> MPQPLVWTQLKQTGTTQPTARSGHTIITVGKTHIMFGGLDNDKNNYKDGKIAPNNQVFTLKLTQNNCEWRQIACQGDVPLPRCYHASCAISADKMLVFGGSYTSNLRFNDTYILKTTSYQWSKPANQISGGEPKNAESKIGAPQPRYGHSATFFEGKVYIFGGHGGINYQRLAFNDLYVLETENFEWTRLEPKGNPPDPRGGHSAAMMANKPQLMIFGGWSFTSQYSNIMIYDIEKDEWVDPEIAHEIPKWNLSGIMAPSIPSWKYFIFGGSVGSFEEGGNRTNSRFVDDSFVLDIDTLSWSSINLEADETSKAVCKPRPRESASIFYDSGESRAIVFGGWANNWLNDLWALNVSTITGPPYAIFSIKPALGPLTGKTKVLIEGDGFKDTQNISVKFSGGKLEKEVNGTFVNEKEISCETPTFDYPRSVEVTVCMNKGDYTITKSAFTYYLNTKADKTIAYGPGLLTENLIGVQTTIVIQARNKNDQNRESGSDEFVVTIRNPAKIKKEEEVKEGDKANTKNTIKEDEEEEGEDEEENKKKKEAEKAAAEKAAAEKAAEEEQGEAVDPSLVPFNIVDNDDGSYFIQFTSEEEAVLEIDIKFKDENNELHSIRGNPFRCGFVKGSKPNNNDLTGSAVMNYISKQLKDIQEFIENTKENIEIRNKNIRENVSELINVMINLEKVRVKNDDDVLTLDTVEEMLNFLKKKDFGKDSDIKKCKKLQEEWKNLAKMAQAVKKDIQNPVKTESDKTKENIKKFEEITLKEYANSLKKESFFIYKTGVSESFKRIGEVKQKVDEFEVQLNQYEDFARMFEFPDAVIGSKKLMEQIRTDVSSVEKLWVRIEISEKTMDEYKKMKWGSINSMDMEDEIKKLRKALTDLRGIDKRSNAFIGITEELKKWATFLPLLGELKDPSMNSEDGRHWKKLKDLVKKEFDVSQELMLEIIWDLKLFDYKDGIEEITDQAKQELKMEKALKKIIDFWRDIEFELVQHKNTDIHTLKMSEENFETLEDHQLQINNMLLSKYVAYFEKEVEKWKYDLGSVYDVVQLLLEVQKTWSFLENLFIQSEEVKRELPNESAQFVGIDKDMKEIMQKGCDIKNCLKFCTIEGMLKRLENIQAQLKVCEKALNEFLDSKRRAFPRFYFVSVNDLLDILSNGNSPAKINRHMSKIFQAIDNLQLKEDSSGGRPTALKMISCVGTEEVDFSSPRLLQGKVESYLKDVIDTMIGTLKSVANSSFKNFQSMTRKEWLKSDPSQITLLVNNIIWSKAVEDCFLKLQSGDINAMKLFLDESIKQLTELIGMVQGDLSKPLRQKIMCLITIDTHSRDVVHRLINEHVRKAEEFQWQSQLKFYWVDNDAKIKIADARFVYNYEYLGNGPRLVITPLTDRIYVTATQALHLKMGCAPAGPAGTGKTETTKDLANALAKACYVFNCSSEMNYESMGNIYKGLASSGCWGCFDEFNRLLPEVLSVCSVQFKAVTDAIKQNVERFIIEGDEISLDPTCGVFITMNPGYLGRAELPEGLKALFRPITVVVPDLELICENMLMAEGFIEAKILAKKFVTLYMLCRDLLSKQLHYDWGLRAIKSVLVVAGGFKRSEPEIAEQALLMRALRDFNIPKIAFQDLYVFHGLLGDLFPGINIKPKKDLDFEKIITDVCIENKLDPDPEFVLKVVQLSELLAIRHCVFVMGPPGAGKSTTWKILAKAQDKTNKKTTLIDIDPKVVSTKDFYGYNLPSKEWKDGLFSKMLRSLAEQPDTNPKWICLDGDLDANWIESMNSVMDDNKILTLANNERIPLKPHMRALFEIRDLRFATPATVSRAGILYISDEVGYQWRSYVKSWIKQEFSQDQEMSKNLDTLFGKYVPDTLDHIKKHCRFLVPVSPISQVISICKSLQTLLKGDVKNLEYLFVYALIWAIGGALAEKDSIDYRKDFSTWWKGAWKTAVKFPSKGTIFDYYVDQSGDSSKFVEWSKRLENKEFDPQVETMGNITVNTIETLATTEFIKSYLMVKHPSLLIGNSGCGKTQLAKGILKEIVQAKPENYAYQLINFNYYTDSTYLQGQIEQTLEKKAGRQYGPPGKVQLIYFIDDLNMPQLDAYDTQTAIALLRQLADYGHFYDVSKLALKDIINTQVLAAMNPSAGSFFVNPRYQRHFWTISIPFPDNESLSLIYITFLNGHLKRFKSTIQEYSNIIVRASLMLHQAVTQNFRKTAINFHYEFNLRHMSNVFQGLLLSDPNKFTEPDKLIKLWIHECERTYGDRLVSTDNLKTYKENIFDIVKKSFSKFNFSRYFGNNPENLIYCNFIAGINSDRFYDQMPNNEMEKHISEALKEYNDNNAFMGLVLFEDAMKHVCRICRIVLPSSGHALLVGVGGSGKQSLSKLASFIMGYTTFSITISATYSMVDLRNDLQQLYFKCGPKEEGILFLFTEGQITNERFLVYINDLLSSGEIAELYTLDEKEAMINQVRAKVKGEGKPDTRENCWNWFIDQVKKNLHMAICFSPVGDMRRRARQFPALVNCTVIDWFQPWPYEALFNVAKSFLEPVDLGDDKVREAVVKFMPFSFTLVNDLGLKLLEQERRYAYTTPKSFLELISLFTNMLAQKRESLERNKERYETGLVKLKETAEQVAIIEVEVKEKQVEAEAKKKEADAFAEVVGREKDKVEKENSKATIEADKCGLIKQNVEAQKSSTQQDLDAAQPLVEQAKSALNSISKKDFQQAKSFASPPAGVPEVFAATIYLLAGYFNEAIEIDKNKKPKDVSWKSSLKLMKSPEEFMEKLLNFKDVVDANQVPAANVNIVKNQYLNMPSFTPEQMASKSAAAKGICSWVVNIVKYYDVIQDVEPKRKALKEATEQLEEATVKLNEVEEVVRKLNEELNKLKAENDKAIAERNAAISEAERCARRLNLAQRLVTALSSENERWGKSIIQLEDQLKLMVGDVLVASSFVSYSGPFNKKFRNIMINQNFMKFMKEHTIPMSPDPNPIKILTDESTIALWNKQKLPSDSVSIENGTILTNSARYPLMIDPQLQGITWIREKEKANNLKILRLGSKNINRDLELSIENGYSAIIENMNERIDAILMPIIARSFIKRGKNKIIKFAGKDLILHPNFKLFLHTKLSNPHYPPEIQAEAALINFTVTEAGLGDQLLSLVVARERPDLAKMKIELITQQNDFKIKLKDLEDELLYKLANAKGDILDDIELIENLEYSKKLSVEIAEKVAAAKITEAKINETSENYRPAASRGALFYFLLSDLSKVHSFYKYSLESFIVVINRAIDAISENKIYGKTTMVPYGDETYASNQHEKEEEEEEEEHQQAQQQQNQEEQQEQKDEENKGPVEEEQPEGENKGPVEEEGAEGQNEGPVEEENAENQEGEGEEEGEKQQKAKDSDEPMSPRSLKKRVDELIESLTYTAYQTTRRGLFESHKLIVAAMLCLRVLLRSEELNSDEVDHLIIGKVDVNPTPMPDALKSFLNDNIWAACKALETIHQFQGFCQSLETDVLQWKKWYSEEKAETADLPKAFKELSKFHRLLLLRALRPDRLPSALSQFVHDKMGERYIEQPPFNIFETFQETSKTVPIFFVLFPGVDPTPDVERVAATFDVSANNGRFINISMGQGQEDRAKKALFDCAQKGHWIMLQNVHLMQSWLYGLNGLEGFLESVFASPKTHPNFRVFISSEPPNVLLPLMQIIPESILQGSLKIANEAPQYLKANLRRAYNKFDQEFLDKCDKKPTEFKSCLFALCFFHSLMLGRKKFGTQGWSRVYNFNDGDLTICADVLYNYLSKYDQVPWDDLRYIFGEIMYGGHITDDWDRRTNRTYLKVLIRSELLQQNFNLAPQFKSPDPSKFDYEAYRKYIEEKLPIESPQMFGMHPNAEIGYLTQTCDQVFNTILEVQGGSSGGGASKKDDGVMVTLTDFKTRCPHDFNMLLIEEKVKEKTPYIVVCLQECERMNGLLKEIKTSLEDLRLGLTGALNMTDAMESLQQSLSFNKVPDTWEKKAYFSKKPLSSWFADLIERNIQLQEWCKELVTPTSLCISYLFNPMSYLTAIMQFTARAQGLPLDGITIQTNVTAMKGPEDVVNPAENGAYIHGLFLEGAAWEIGGQGQDGYLIEQKPKELHPKMPVINAVAVPLDKKKKNGQYDCPTYVTSARGQTFVFTANLNMESDDSDPNKWILSGTCMLMSDD;> MGDHSQKDSPEDFIINRLSQALGIQKEKIKKSLETQQDDKGEVTNKDEFQGFIQQDNSTNILWVSGQSEKCTFYYGQLPPIDKFKKKGIAVIKLGLHKLTNENVAKDVVVVEITNNLLEHLNSVFNEIMSPVMQNPLNQQGWTDLVAKDLMEKFNNYVAQVYVLLGQIKGKTMLPLPSHKLTSSDTTPDKDKAHVFEGSIITWTKQIKNVLKLEPEQLLKYGNDPGPLAEIEFWQNKRDNLNLIDSQLKSVEVQNILHFLDNNKSTYTTPFTKLQAEVKKARLEANENYRYLFTLKDLFSKLQESQPSDFPTLYELFIPIMHTILLIYNKSKTYNQPPRLVVLIREICNAIISNAQAFVDKDTIFSLIDSKETTEACDKLQVTLDVCSKFKDAYFEYKAKAGGNWKLTSNALFVRLDSFLERCQDILHLTNTIVQFNKLEKIELGGTKGKTLTESIAQIFKEFEEAVQAFTSVSYDIMNIAEKKFDDDFYEFRSKIKELERRLASVITQGFDDYDTIYGRFKLLDNFEGLLTRPIIADELEKKHIVLLEMYKQDLKQVQSIFLEGKQFVDSMHENAPLFLNMPPIAGALTWCKSLRDRIQEPIEKLAQLGQGITEREEYKDVQKLYTSITKSIKDYEDQKILSWEKEVEDSSQDKLKQTLLCKDENDLIKVNFDPSLVRLLKEVKYFLLLRLEVPTTAKDIYTKAETYRTQIVALDMIVDNYNHIKTCLLPVEEPLVKKKIQDMEEEVKPGIEEIRWKSTNIDQFISKSKSIVDQLFETVNKMKDSLQKIHKSLANFNVKIIERKNRPMSPDDYDQFLKAIFSNKLTIVKDNGNQIQKLVKEVLDAVKADKKQNSWKNYNDYVNVIVIEGISTAIQTALLHLNEQINPVFIKRNDISPLFDIRLELGQSGIQFDPEIGESSNQLTVRNTIRNWINDFFNIAGTIQRLDTTMPGDFLQEIRSFFEIKQCLAMITQNLEWIENECNQFRARFDTYSYLWTEDEQISFNRFLDENEPKDEDGKGGDDDEGENTEKQNPLLKGCRAKIPNLDLFDEKITHLKAIQQEISRIKTPEDISWLRINLQPMKTALDARVTRWIRVYTDFLVNQFRTTQKNLLDFIEKTKDGIKKNPADHENLHDKKLLMSVMKVISDVKDVEPRREGIITRMKEMVTKLKKHNVPITEKGTDDPLQQIDNANSNFIEIYGRVFKVKADIIPLQAEETQNIKRDLDIFMKEVESFRKEFMQKLPFDYTESMGYENINNAYDTIMVYYHKLTAIEGRALEYNNLEKLFELQKSNYKQLKDCMNDLKNLKTMWDAIALIHFQYNDWKTKPWRQIKADILLDTNKTLGTQIKNLPKEIRNFKGYNVIVEKVKNMGTVLPLVSALHSEFMEDRHWSQLKQITGTVFDHNSLSFYFEDILALNLYKYENTVNEIVDVAQKEAKIEKKLKNIEQWWSKQVFEFTEYKETKTFASLDNMMEVLDQHSLDLMGMKSQGKYVEFFYDRVEDWREKLGRVDVVVNEWLKVQKNWKILYNIFLLSEDIRMQLPEDTKVFEGVDKEFKDMMSEVSANPSVVEACTIERRDVLVGWSQAIKKCEKALNDYLEQKKKSFPRFYFLSNQSLLTILSNGQNAPKVCEYLGDCFDGLKTLTFEPPANPAETSKVGIGMISKDDEKVPFSSKFICEGAVEHWLLNLEFRMRETLQEILEGAKNTADLWDSGDKPREEWVEGYNAQIALLTTTIVWTEDVGRAFEDLAGGSETAMKECQKLIEVRLENLIKKVRGDLHILERWKIINIITIDVHSRDVVEKFVIQKVSEAESFAWLSQLKFYWENKPDSDMHLRQTLRFPWEKDKNKNKCIIRIVDWFRFYSYEYIGNAIRLVITPLTDRCYITLTQALNLTMGGAPAGPAGTGKTETTKDLGRAIGIPVMVFNCSDQMNKDSMAQIFMGLSQSGAWGCFDEFNRISIEVLSVVSTQVKCVLDALKEKKTKFSFVEEGEIQLQDTVGFFITMNPGYAGRTELPENLKALFRSCAMVVPDLALICENMLMSEGFTMARVLSRKFVSLYMLSRELLSKQKHYDWGLRAVKSVLRQAGKLKRGDPDMPEDPLLMRALRDFNMPKIVTDDKVIFRRLIGDLFPKLDPPTKQNPELKKIVQDTTKKDMGLVAEELFVTKVVQLAEILEVRHCCFVIGPPGSGKTCVWKTLIKSYINSGEDAEYDTLNPKAVTSDELFGAYTKTKEWKNGVIAVIMKNQVKNEEKYKATHMHKWSVLDGDIDPEWIESLNTVMDDNKVLTLVSNDRIFLTPQMRLIFEISNLRNATPATVSRAGVLFINETDIGWMPYMNSWLERSQINILKQQKEMANMPEYPVIDDVAKSVFYRCFQSYFEQNIDVHDKNRVRHICPMVDIAMIQTICTILDALLIQHLPKLKQMKEEDEKQALEAFFIFAGLWAIGGPVGGGQDDSKDMKEFNTVWKGAAKVKFPEQGLCYDYYYDINENKWNTWKVEDYLPNDQPLFSKIYVATIHTTRLRYMIDIHLQRRKPILFIGSAGTGKTAVVRDYLNSTRPEQVSHKTINFSSFTDSLALQKNIESMVEKKNGRNYGSATNKVLICFIDDFNMPYVDKYGTQSPIQLLRLILDYGSIFNREQLEERKFLQDLLFFGCLNQKSGSFTVDLRLQRNFSVFSMYTPSSDVIKTIFGSILNAHLSTIDDKAQKMAFKLVEATYFTFDKILKNTTAFAPSAKRFHYQFNFRELARVCEGICRTTPGQYSGGDQGKLVRLWAHEMKRTFEDRFIANEHVEFFRRYLTEAISKCIGEFPETENPIAEPLIFTGFVAAHQGLDQQYTQCTIPVLKRVLDDKLEEYNEVKAQMNLVLFQQAMEHVSRICRILDMPGNNALLVGVGGSGKQSLCRLSTFINGFEIDQLVVTASFTINDLRNNLQEIYKKIAKPNSIARVFMITDSQIKEEQFLIPINDMLNSGWIFDLFPKEDMDSLVSGVRNEAKGEGVDVNNLTALTSYFLDKIRKNLKVVLCFSPVGDTMRIRSRKFPGIINNTSIDWFHPWPHEALIDVAFRFLEEIEFPTEEIRQSISLNMAKVHSSIDTANEKFLKLERRYNYTTPKSFLELIDFYKKLLTEKRETIQRQIQRYEMGLNILAETQNKVQGLQEELKVKMVEVNKQREETDILIEKVGKESALAEEEQTIANAEEEKTNVAAAEAEKISKEATEALAEALPALRSAEAAVDCLKKPHVTEMKNLGSPPAGVIVTARVVLILFNQGITLNDPDEKVWKKAVTFMNNPQAFIDKVKSFDGENIEPNIIEQSNKIIQDPSKKFNEKDMAGQSYAASKLCAWAVNIVTFNKIFKQVKPLQDAQKQANEILEEKKKELAIVKQRVAELNARVNSLKRQLEEAEARKMIVEQDAARCQSRLSAAENLVNGLAGENKRWTQNVKFLKENIKSMIGDSLLASAFVSYIGAFSAKLRLELWKNTWLPDIIEKGIPITEGIEPLKILTTEAIKSKWKNEGLPADPMSLENAAIITACARWPLIIDPQLQGSTWIRGKQGENLTTISLSQPKWLGALTSSISSGRAVLIEGIQQEIDATLDPLLQRAVKKNGNQLQLEIGGDPIDYDPNFKLFLMTKLINPHFRPEIAAQCTIINFIVTESGLEEQFIAMVVNIEKNELEMAKQDLVKKQNEYAVTLDKLESDLLQSLSEADPATILDNTELIQNLDKTKKTTIEITEQQQKAKVTEAEINIQREHYRVVAAEGSMLYFLVISLSVMDHMYQYSLESFITFFFKAINRTTVRDENRIPTLILNIRQTIYQWISRGLFEKHKLIFLTLIVFRLMQKKIIDVAYEVAEMDFLIKCPARPGVENTLDWLPNISWDQIQGLINLEEFRNFAHQLEKEAPNRFKDWYNELQPEDQKLPLDWKRLDSMPFKKLLVLRCLRPDRMTISLNNFIRAVLPQGDAFVEMDQKLAFSEILESVINEDSESTIPIFFILSPGSDPVKEVEKIAKKKRIEPGKNFFNIALGQGQDEIARRRIEEGNKEGHWVMLQNIHLMPTWLIELEKILDSYSGEAGGGNSEFRLFLSAEPSTGIPIGILDRSIKLTNEPPAGLKANMKRAWTYFSKEEIEDKDPKIKSILFALCFFHSTLIERRRFGPKGWNMSYPFNMGDLRDSYLVMNRYMEQNQGGKVPFNDLIYIFGEIMYGGHIVDDWDRRLCNSYLFNTMHEQLFDELELFPYIEGKGLSFKVPGQNPYEKYIEHIETSLKQETPLAYGLHPNAEIGFRTDQCKTLFNTLLELMPKEQSRDEKSSDIKSSNEMASDLIKQLLEDSELKNKIFNMEEIKNKIDAENKGPYQNVFLQEIEYMNALLSEIVKDLEEIGQGLSGLLTVSENMEMIIESIALSRVPASWQKLAYPSKRGLQSWLANLFQRIEQLNIFRDDPYSIPRVVMISRFFNPQSFLTAIMQVISRAKAYELNKLYIQTEITKRSIEEIEGAAKEGAYVYGFILEGARWDYQLGQLEESKPKEMFSVLPVTYCKAIPLPPEGKEDKSLYQCPVYKTEDRGNTYVFTAQLKTRFPPRKWILAGVAIIMDVEGVSDEVKKDKK;> MLSSKYSKRIAWMKTTICDSLQLKDMIVEESFQYEKNKNLLEQFLSGEGLNKIFAYYQVQEQAQNDDIKDTGAQDPVLFFTTGDLEKIQDKAVWFLRITNPADDKKKASQQDGNDNDIIFGEITPNTVPMLNALMESVYSRQIDHIITEKIQFWGVAEEEQVLEFQQHSNKFSSEVREAINLMSPGTEHFKLDYEAISGLSESEKMQHYEMKFNEWINLISSQLNDDSEVRKDEKDAGPATELIYWRSRMQKITNWSEQLKSKDFQIVKASLQRHKNHDNQRPRGDESLSKLMMEYNRLDLLLTDKLNEAKDNVKYLTTLEKFIEPLYNGTPQQIIDTLPALMNAIKMIHTIARFYNTTDKMTGLFIKITNQMIKNCKDRILNKKDNGDNPSLYKMIWEQDPAELIEVLGSCIKLYCEYKKCYNDTKEKVADMPKGKTFDFSDAQIFGKFDTFVRRLQKLIEIFSNIQQFNALAKHNLEGMDVLTNKFKKIIDDFKKKGHNLLDTANNKFDRDWVEFNVEISHLDGELQNFIDNNFNRFRNIEYSLKLLHKFQSTIKRDSLKHNLTSRYNAILHNYATELDTIQRVFQDQKSNPPLVRNMPPEAGKIIWARHLFQKITGPINIFPENVINSTEIRRYYGSYNTLGKQLTIYEMWFYQDWVNKIEQSKAALQATLIVRHDENKKLYVNFDLEIMQLIREAKCLDRQGIEIPESARIILLQEDKFKTYYNELLYALKEYERINSKIKPICKNLLLPHIEDLDLKLRPGMVTLTWTSMNIESYLYYVHQGLKKLEQLIINVNDIIENRIENNLKTVSKVVLVHLPQDTKPLSLDSFVQLQEEYINSKTDFLTSKNVEVERAVDDLLQTIMLYPLDPHVDPVLPEETKRIKRYYFWYFYQALLNSTQNSLNAMKYRVCGKKIPGANTLQNLKPFFQVEVQLNGDKVTLNPSLQEIQKSINRAATAVLRCSKHLYNWDQQNKDSTDKATFYDMIACDKEIVKVILLLTGSIQGTKNKVNEFLSGFTKFEWLCKESIQESIKKFSKNGPTLQNYEDQLKKFSQIEEEIEKIVPTYKIGAMELMTHNICTSLSTWAKEWKLQYSQDLHKRARQLLDSLTEQTKMLSTKLSKPVKDIDSLGYVMETLEQIRKEQAEIDMKFNPVQEMYSLLDNYLPGGITDKDEMDARSLLRRNWDILIQQAEIKGKEYQHKQAIYLKELKQSIKDFTNQVSIFRRDYEKNGPMVEGISPAEAMERLRRFEDEYDVKYQMYKINARGENLFGLQNQKYPELEKTDAEIKNLNKLYNLYDSVIKNIQQFKEKSWQDVSKDDLAKMEEDAGKYGEQCSRLPKDLKEWQAYRDLKNYIDSLREQLPLIISLKKPSIMPRHWEKIKEITNTKLNYENPDQFYIEEIMGAKLLDFREDIEDITESADKQLKIRTGLDEINLYWNDMQFQFGIWGKRDVPCMLNGLIVGTILERLEEDQLQLSTFNSQRHVTPFKAEVENLIRTFSDVNDTLDMWVKVQKLWTSLEPVFTGGDIARQMPLQAKQFQGIDKNWMKIMEKAVETKKVIPCCQNDMLKDFLPDLNRKLEDCQKMLEAYLEGKRKKFPRFYFVSNPTLLKILSQGSEPTSIQEDFEKLFDAITKVTFESAKDKKNPALKQITQIQQVIGRNEENISLTGYYVKCEGNIEDWLKKLEQNMQQTLKDIASAAAQQVFQVGLKEFVSSQASQIALLGLQILWTSKVNEGLERLSRNERNAMDIKRNEIKEHMNILSSMCLEDLNGAVERTKVETLVTIQVHQKDISMDLKCKDVNDFEWQKQTRIAWKTDIDECIISITDWDSPYSYEFLGAKERLCITPLTDRCYITLAQAMSMYYGGAPAGPAGTGKTETVKDLGRTLGVFVVVTNCSDQHRYRDMAKIFKGLVQSGLWGCFDEFNRIDLEVLSVVAMQVESITTARKQHMKKFMFPEEEIEIELIPTVSYFITMNPGYAGRQELPENLKVLFRGVSMMVPDREIIIKVKLASVGYLQIDLLAKKFNVLYRLCEEQLSKQRHYDFGLRNILSVLRTAGNTKRQEIKSDEEMLLMRSLRDMNLSKLVADDIPLFNGLLADIFPKLKEVPKKLYPDVEKKIPEEINAESYLINTPSFQLKIIQLYETCLVRHGFMLVGPTGSGKSTIMKILTEVLTKLGSPHKIVIMNPKAITAEQMYGVKSEISDDWIPGVFSTIWAKSNNRALKHTTWITCDGPVDAIWIENLNTVLDDNKILTLANGERIAMTENCKVVFEVENLNNASPATVSRCGQVYVSPTDLGYEAVIEGWIRNRKASGRAEESDKLGNILRKYLINMRFIELQSKECKEPMMDTSPVISVINILNLLTGCLQYFVQTQRTLSEQEYEKFIVYSMAWAIGGIYEAQDRVRFHELLLAKNAPIPQKGKENETVFDYYVSQDYLDWKICSPEEWVPPQSLQFSQLLLPTLDSFRAEMLLNFILTQPKSHTCSNSALLIGGSGTAKTSSVLLYCNKFDPQKMLFKRTNFSSATSPFMFQSTIEAECDFKVGKEFAPPGNKMMTIFIDDMSMPFVNKWGDQITLELVRQLIETGGFYMLDKTQRGNQRKMKNLQYIGAMNHPGGGRNDIPNRLKRQFFIFNMILPLSIEGIYGPIIKHMFKQKYFSDSTYKVIESLTSATIALWNKVKSTMLPTPAKFHYVFNMRELSRIFKGILTCKKDTINDAPKSMKIKPELFLVGLWRHEAERVLADKLVNNKDKDTVMGYIQEVSLESFSQIENEILEKYSSEKTFLFCDFLRPDVINEDGIIEEEAPKIYEAIDSLTELRKRCNFLLSFYNDRNPSKKMPLVLFDDALKHLLRISRIIRQPRSSGLLVGVGGSGKQSLTRLAGFIGKNLIQQIIVTKTYSDKDLKEDIKKGFDDAGHLGKQVTFLMTDSEVKKEEFLEYINMVLSTGEIPNLLAKDEREVWLGDISQAYCKEKNLGNIDPPQSELWTYFVDRVRDNFHIMLCFSPVGQKFRERARKFPALFNECTIDWFLPWPEEALVSVAETFIKNFDKLDTKEETKQELMKHMGNVHLMVNEICDEYYQKMRRQVYVTPKSFLSYLNSYKTLYIEKYDELDQQEESFKIGLNKIQEATITINQMEISLKEEEIQLNEATEKTNQLLANLDKESKKANQKGEEVAATNKQCEIQAEQISKEKEEAERELEAALPALRRAQEAVDSIESKDIVELKANKKPLDIIKYIMDAVLVFFKARLIPIQIEERVFNKKEGKAVLFLKESYDESGIQTLGDMNFMKKLKEFEKDSINEETIELLEPYLNQSEDWFNDTFATKASKAAAGILKWAFAIYEYHQKSKIVKPKRIQVAIAEGRQAIALKELEKAREDLAQIQAYIKNLKDVYTKQMEEKNELEMKAAKTKKKINTARTLITSLSGEKDRWGKGAQDISDQKRKLVGNVSLSTAFISYCGPFNAEYRNKLAQQRFVVDMKKRGVPVTPGLELTSFLIDDATIGEWNLQGLPKDDLSIQNGIMVTNSARYPLFIDPQGQGQNWIRNKLSASIIPERCITTLSHPKFKDMFLKYCMESGLTLIVENIENEVDPMMDPVLERQIIVKGKTQFVNVAGTEMELSKEFKLFMTCRLANPSFSPELSAKTTIIDFTVTQSGLEQQLLGKVISKEQKALEDSLNQLLADVNQNQKDLQRLDKNLLERLINSQGNLLDDTELMDVLNNTKTQAKEVAAKLIDAEIKTKEINEKREQYRPVAIRGSAIYFTMIEVSLVNWMYNSSLEQFLKLFIESIDLSEKAQLPSNRVKNIISFLTFHVYRYVNRGLFEKDKITFILMMAFKILTTAGTISSGDVSLFLKSGDALDIKSERQKQISYLEDNQWLNILALSKHTFSGQTLPFFKELPDLISRSENQWRNWIDKNDPENFPIPDFAESINQEKEIGSFISLCLVRSLRNDRTLIATQNFISNVLGKEFTDPISYPIEGIWQESSNMDPVLFLLSAGADPTSSIDELAKKKKKFPCEKVSMGEGQERVARQVIMKGFVEGGWVILQNCHLGLKFMEEIETLVSPINQIHEDFRLWITCEQHPKFPLGLLQKTLKVTNEPPKGLKAGLYKTFTTIITQEFIDKVDHSNWRSLIFTICFLHSIVIERKKFGPLGWCVPYEYNYSDLEASLLYIEKYLTNLMSTPQPNSHNLPISMNVVRYMICEVQYGGRITDDLDRELFITYGETYLKDGIFGNDYFFYDIMVDGSGQKFKYRIPQNPSAELIKYQEYIAKVPTVDNPEVFGLHSNADLTFRLKESKEMINTVMETRPKDSSVGGGKTREEIVQDKAKDMLKNLPPDYNDVEVRELVSKLGGPNPKTSTERGMTVPLNIFLYQEVTRMQRVIGLVRKTLQDTILAIDGQIIMTPEILEAINAIYDAKVPNSWLYDPSGAEISWLLPNLGSWSTSLSDRNKQLNDWLRSGQRPILFWLTGFFNPQGFLTGMKQEVTRNHKKGDGKGGEAWSLDDVVYSTTVKEREKEKDIEQPPAEGVYIKGLYLEGCKWSKNGLDDSDPKKIFADLPILHVSAINKKKTNEQDRMSNTYLCPVYKYPKRTDKYLIFRVGLPCEGSNNPSHWKLRGVALLCSTE;>MPPKQTKVVASRKTVMPISRAGRAQIRRKDSNTQNNMNDQGMEDEEIDQQREGMKNQYEQLTAQELNEDMPSKMLEPKNPQAPKNITVYDYYTRKFKTDELVDQMIVHFSMDGDYIWKESNEYKTQEEIRDTKKALIKEAMRKQESEEPGANHDEEAIKQTLRNKFNYNTRECQTINPSIRERGVSTEPPPSDTICGNITQWEIFDAYYAEIMKDHQIENKKKKEVDQDKKQDQSMYSTSFKRCCKIMERMVVQNDQEDKYHDYRYYWSQGDNLEAGKNEGHLLPIWRFSNEKQRKKNVTSICWNPLYPDLFAVSLGSYDFTKQRMGLICLYSLKNTTHPEYAFNCEAGVMCLDFHPKSAALLAVGLYDGTVLVYDIRNKHKKPIYQSTVRNQKHTDPVWQVKWNPDTSKNYNFYSISSDGRVMNWILMKNKLEPEEVILLRLVGKNEEESTLIGLACGLCFDFNKFEPHIFLVGTEEGKIHKCSRAYSGQYQETYNGHLLAVYKVKWNNFHPRTFISASADWTVRIWDSKYTSQIICFDLSMMVVDAVWAPYSSTVFACATMDKVQVYDLNVDKLNKLAEQKIVKQPKLTNLSFNYKDPILLVGDSHGGVTLVKLSPNLCKSGPEIKQTEDKKAMEEFKNVKIEDYEREKMENLLAVVSKWEREDA[2x];>MAEYFTYSKKRKEFNNPINFQDTETRYGGIQNQVVNINQYVQRNPNFIDLDNIAELSEHSVNTERVKTGDRGMSHKEGGWPGNVDPNEAQETGRFKKRIEKDTSFPQAVKDLKEGVEKCIYQNNQIDLLEEYFEGETSEHVVENLSSKTLMLFKDEKEICKRSVSEISWHPEGPTKVAVSYAIMRFQQMPEKMPTQAYVWDLLNPNSPEIKLMSPSAVTNISYNQKIPDQIGGGCYNGLLAVWDGRKGENPIMISPVENSHYEPVTHFHWLMSKTGSECVTTSTDGKVMWWDTRKFEAGPVEKLNIIEGLGENEEIIGGTALEYNVEAGPSKFLIGTESGSILTANKKLKKPVEITTRYGLDQGRHLGPVYSINRSNQNPKYFLSVGDWSCKIWVEDLKTPIIRTKYHGSYLSDGCWSPTRSGAFFLVRRDGWMDVWDYYYRQNEIAFSHKVSDSPLTCIKINQTGGAYHNSGKLCAIGDQDGTVTILELCDSLYTMQPKEKDIINEMFEREYRKEKNLETIKKQQELAKRQVQKDMGSQKEKWEKKKLEMIETAEASFHENLAKNPVNEEEFNELDSPSEKRKKTNQNQGREQEEQSREEQEASGNFNQQQQQQQEEEQQQEGEQQHHQNQEHQNGQGHENGQEEGEENGEEGNQQENEGQEENEQQQE[2x];> MAQDINADDQLKQLSALEGANGYVIFNESGIPLKRHEKSISHEKAVHIAALVSDLWNVSKKVIQRDLKTPENDIEVIRLRTKHSYEYIITQSGDFTMLAIQLCGKAIEEAKKAAAAAAAAAVVQEENKEKEKK;> MSEVEDTLNRIKTHKTVLGYLIVNSEGGVVRGAFKDEEESKNIANSIPLLTKKARSVVRDLDPTNDLVFLRIQTKLNEIMVAPDDEFSLIVIQTKGEKRDEND;> MSHLDKVQPVIKNSDMSVEMQKEVEEVAKKAIDYCNTDKEIATFIKDDFRSRYHGTWHCIVGRNFGSFVTFERSYYIYLYVGQLAILLFKTG;> MEQEKAVTDMDINELRKLMIGKAIINSSDMQGDLLQEAQDVIQSGIENNSAPVLNIEAACKYIKENLDKKFGPTWQCIIGEGYAYDVTVQNNTLLFMFYNGNLAVLIFKS;> MGDHANEQIIDMPENSEMKSMKNDAFSQAKFAVENYKFENKISSHIKKFFDEKYGPNWHCVVGKHFNAYVSYDSKNFIFFYEGQLAILLYRKG;> MASNQQQKEDPKEQQQQYKTFMGARVLWPPECADDILEGAIRETQDALKKFEIAREGQKIAEHLKKYMDDHFDPYWHVFFGKNFGCQAVHNKNRFIYFYIEKTAFLMYQTQ;> MSDSDSDEGRVVEEPLPPHIIRFNDMAQHLLKKVIRQADVLIKENPQGLEKDIALNLVKFVKSQPEFKIGDGEWQCIIGKNFGCSLTFDANVLAFFDLLPSRKSILLFKSG;> MNHEPEVKATDMEEDMIKRVKEIAINAVKEYKQEKQIAHYIKYEFDKIDGYGWNCIVGRNFGSHIIHQTKKYIFFKINELCLLLWKA;> MKGTYLYLNIYKRKREASLITLNYIKNRFYPSKIQKIIKELFEDRLKGVEYDPNNANQLSERLVLELREKIKRGKVPRYKIGVQVVFGEIKGQGLRIASKCLWDVQNDNYASYTYTSEKVYCTGIVFGCYFE;> MGDTDKEYISEEVQKAIDDSVKQVFGIKDDSSQVTITYNKDKVNLWTQQIIDYTIRGLNKLGKHFKYCVTAILQQTNHAGISVQITAYQDTNTDGSLIQCYEINDIYAIVSVFAMAV;> MSHPYIEITSTKQFEDILEKNEYVLVDFFASWCGPCKILAEQFEPIKKDHKNLTIVKVNIDEEDLESIVESHNVSSLPHVFLYHKKTVVKQFIGNQKDQLWEMAKLSDAK;> MFNFFSSANINQNIPKYSVNDFVFRLKKIEKIVVKEGLDGFLLINGVDSRENTEYVKLTNWLFLGNSGLEIEENEYLNQIYSDMIVLIKKGTTHIFIDPEALNSLQTLIYSIPNVDVFCPTEKQYEDKDEMELLKMAFFLRVMKPTKKVGILLGQKDKGKINSIEKWPLIQSYGLEELGVGFFSMNHEVVDLTLRLNAVYKNYDKFFVSKLIYVVAKRLTGHFNSAAGQLGDMKMHKRNLATESQLTEIFRDTYEIEEISKWVQIRGVNAALPKPRVLFGKNTSADCSKEPSVAPLKDLKYSETFHSFHATFETFDLRTCLRAARTYFLAKGVKEERNLITLNDDEGVPQGYELNIDENQQYKDQDFLANLYLSIIIGFNEVMQLITKDYKNMTEEFIQDYIFQKVSKVYAGFQIPESEITLDKIQIILKAYNSFGEEVKIDFKDTISFKLTPYFFMVRIEQKNIKSQILNNTVLGSLVFAESFILQEGCYLLLTKEIPYFDLWNCQNDYSEKIEKMKKRILWEPLGKQISDELPKNRIFVQTGRKSNYGFDIPIMQASYYMHELGLRIETQRLGWFILFFKEMKEIQITQKMNHTWLIFKVDSNITFNSISKDTIALEFTGDALEQSFFKIKNYFEENQIKYEYQVDIPAIFQESQIAKKQILNQQSQGQKLITMNSIQNEQFFISYIESKQLMILNQMKDLKLSAYKNLYEQMQISQAITPVENHIGVILVNGSYCSGKRKFAENLIRFGSDNNLRLHLYKFDLNEMSELTEKSYLSGLLKFASEKKIQNTDVIVASVPHFINTKILIDYFSKSEKISNAFYIRTIATKININNIYSNFNKNPVNNVFTYGVEGYSQFLLLDTYNNYDADVNALNKTLSGVLPGAKIYKIMNNILNPALAKDILTSITFISEQNNLNRLKYSVQYDLLTSNGPSSVVFIPFKLPILREKIRDLIYKKILQNGNQTLVDTIEAEQKIAEFKELNKNSKDPLMIEIIKLKEKIEIQNAQTSDQAIKIDYVKGILRYDSKLKEGLEEITITPNYFIERTVKG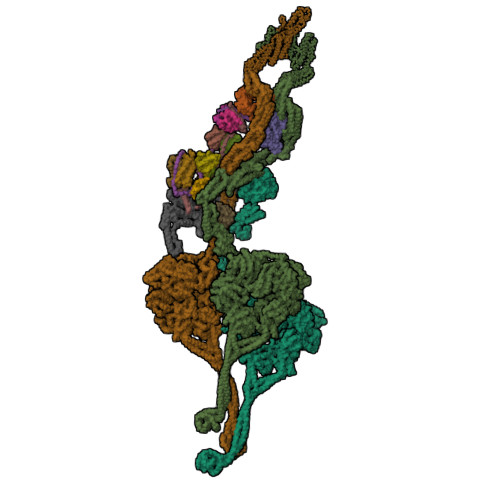VDAKEFTEELNGVSFKNVKYTGITNSIINDMGFVFAGKNLNKEKLLELLYKLVKPLNKQKLRQRKDLTEEEIVDIQFRNRGEGLENGEFYDGQFWRNIQGLILPHHPKKDEFIEEYLKQEEVRINQINEQLQQEWETWKQVYDKIHLDK>[5x]GSAAAQDMVSPPPPIADEPLTVNTGIYLIECYSLDDKAETFKVNAFLSLSWKDRRLAFDPVRSGVRVKTYEPEAIWIPEIRFVNVENARDADVVDISVSPDGTVQYLERFSARVLSPLDFRRYPFDSQTLHIYLIVRSV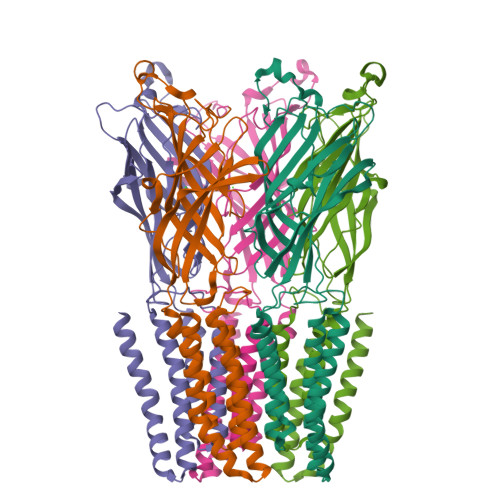DTRNIVLAVDLEKVGKNDDVFLTGWDIESFTAVVKPANFALEDRLESKLDYQLRISRQYFSYIPNIILPMLFILFISWTAFWSTSYEANVTLVVSTLIAHIAFNILVPTNLPKTPYMTYTGAIIFMIYLFYFVAVIEVTVQHYLKVESQPARAASITRASRIAFPVVFLLANIILAFLFFGF> MKESYYSIGEVSKLANVSIKALRYYDKIDLFKPAYVDPDTSYRYYTDSQLIHLDLIKSLKYIGTPLEEMKKAQDLEMEELFAFYTEQERQIREKLDFLSALEQTISLVKKRMKRQMEYPALGEVFVLDEEEIRIIQTEAEGIGPENVLNASYSKLKKFIESADGFTNNSYGATFSFQPYTSIDEMTYRHIFTPVLTNKQISSITPDMEITTIPKGR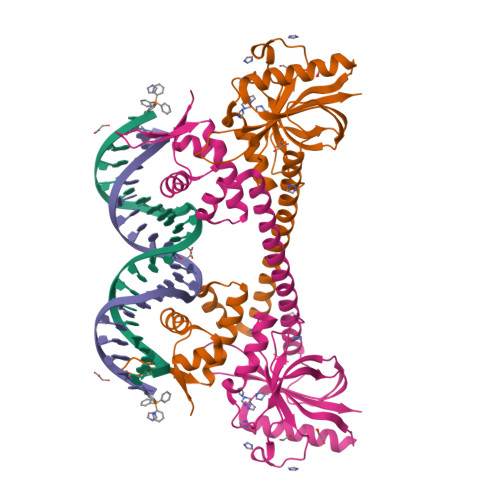YACIAYNFSPEHYFLNLQKLIKYIADRQLTVVSDVYELIIPIHYSPKKQEEYRVEMKIRIAE> GSDNESDEEVAGKKSFSAQEREYIRQGKEATAVVDQILAQEENWKFEKNNEYGDTVYTIEVPFHGKTFILKTFLPCPAELVYQEVILQPERMVLWNKTVTACQI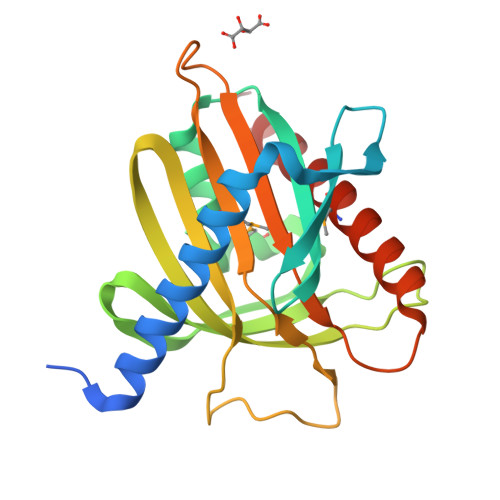LQRVEDNTLISYDVSAGAAGGVVSPRDFVNVRRIERRRDRYLSSGIATSHSAKPPTHKYVRGENGPGGMIVLKSASNPRVCTFVWILNTDLKGRLPRYLIHQSLAATMFEFAFHLRQRISELGAR> AQSVPYGVSQIKAPALHSQGYTGSNVKVAVIDSGIDSSHPDLKVAGGASMVPSETNPFQ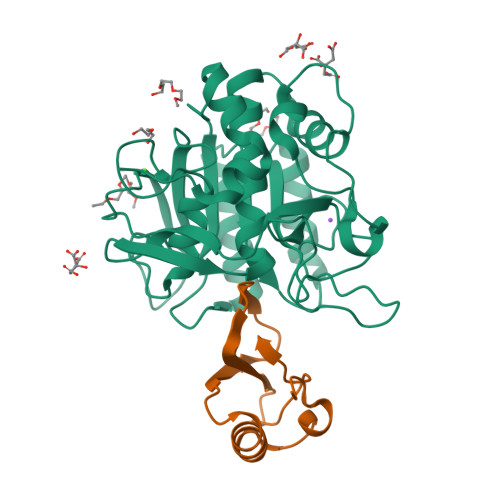DNNSHGTHVAGTVAALNNSIGVLGVAPSASLYAVKVLGADGSGQYSWIINGIEWAIANNMDVINMSLGGPSGSAALKAAVDKAVASGVVVVAAAGNEGTSGSSSTVGYPGKYPSVIAVGAVDSSNQRASFSSVGPELDVMAPGVSIQSTLPGNKYGAYNGTSMASPHVAGAAALILSKHPNWTNTQVRSSLENTTTKLGDSFYYGKGLINVQAAAQHHHHHH;> MKTEWPELVGKSVEEAKKVILQDKPAAQIIVLPVGTIVTYEYRIDRVRLFVDRLDNIAQVPRVG> AASPPTEEAVVATEPLTREDLIAYLASGCKSKEKWRIGTEHEKFGFEVNTLRPMKYDQIAELLNSIAERFEWEKVMEGDKIIGLKQGKQSISLEPGGQFELSGAPLETLHQTCAEVNSHLYQVKAVAEEMGIGFLGMGFQPKWRREDIPTMPKGRYDIMRNYMPKVGSLGLDMMLRTCTVQVNLDFSSEADMIRKFRAGLALQPIATALFANSPFTEGKPNGFLSMRSHIWTDTDKDRTGMLPFVFDDSFGFEQYVDYALDVPMYFAYRNGKYVDCTGMTFRQFLAGKLPCLPGELPTYNDWENHLTTIFPEVRLKRYMEMRGADGGPWRRL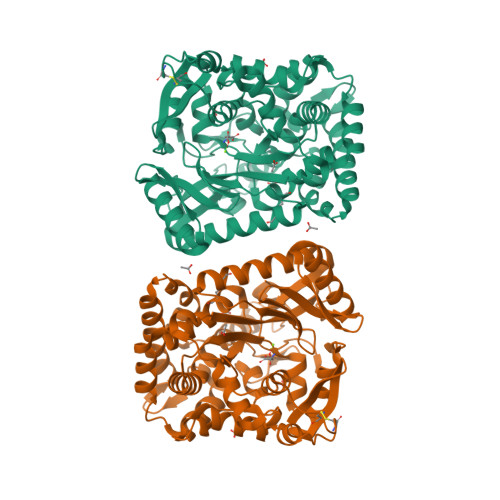CALPAFWVGLLYDEDVLQSVLDLTADWTPAEREMLRNKVPVTGLKTPFRDGLLKHVAEDVLKLAKDGLERRGYKEVGFLNAVTEVVRTGVTPAENLLEMYNGEWGQSVDPVFQELLY> GPLGSPGIPDSARSFLERLEARGGREGAVLAGEFSDIQACSAAWKADGVCSTVAGSRPENVRKNRYKDVLPYDQTRVILSLLQEEGHSDYINGNFIRGVDGSLAYIATQGPLPHTLLDFWRLVWEFGVKVILMACREIENGRKRCERYWAQEQEPLQTGLFCITLIKEKWLNEDIMLRTLKVTFQKESRSVYQLQYMSWPDRGVPSSPDHMLAMVEEARRLQGSGPEPLCVHCSAGCGRTGVLCTVDYVRQLLLTQMIPPDFSLFDVVLKMRKQRPAAVQTEEQYRFLYHTVAQMFCSTLQNA

Protein tyrosine phosphatases (PTPs) play a critical role in regulating cellular functions by selectively dephosphorylating their substrates. The ∼280 residue PTP catalytic domain consists of an α/β structure, and biochemical and structural studies have led to a detailed understanding of the catalytic mechanism (Barford et al., 1994; Zhang, 2002). Key features of the domain include the PTP signature motif, the mobile Trp-Pro-Asp “WPD” loop that in the closed conformation positions the conserved and catalytically important aspartate residue, and the phosphotyrosine recognition loop. Here we report the crystal structures of 22 PTP domains, including two tandem-domain RPTP structures and a detailed structural comparison of this protein family.

In the first category are TCPTP, SHP1, SHP2, BDP1, LYP, PEST, PTPBAS, DEP1, MEG2, and GLEPP1, which have a “PTP1B-like” accessible pocket that harbors a basic residue corresponding to Arg24 of PTP1B. This pocket has the potential to accommodate pY at the +1 position as in PTP1B or potentially other acidic or phosphorylated residues in positions N-terminal to the substrate pY. The new structural data and analysis presented here suggest that a secondary substrate-binding pocket, similar to that found in PTP1B, is present also in SHP2, BDP1, LYP, SHP1, TCPTP, MEG2, PTPBAS, DEP1, and GLEPP1. PTPs with particularly high enzymatic activity against generic substrates were RPTPσ and PTP subgroups R5, R3, NT1, NT2, NT3, NT4, and NT5. In contrast, RPTPσ, the R7 group, and NT4 group PTPs were quite selective and showed a preference for a sequence derived from the phosphorylation site in N-cadherin (pY785), a reported substrate of RPTPσ (Siu et al., 2007).>[7x]MRWILFILFCLLGAPAHAVSIPGVTTTTTTDSTTEPAPEPDIEQKKAAYGALADVLDNDTSRKELIDQLRT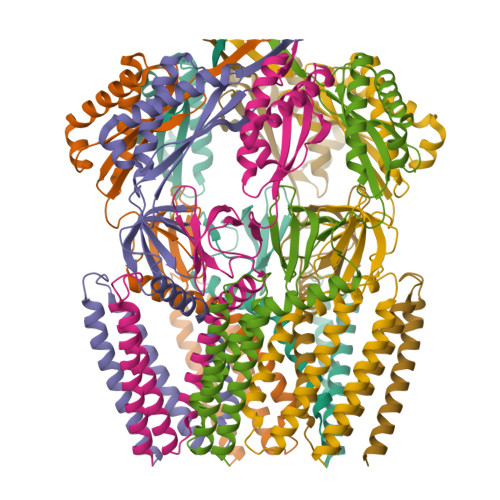VAATPPAEPVPKIVPPTLVEEQTVLQKVTEVSRHYGEALSARFGQLYRNITGSPHKPFNPQTFSNALTHFSMLAVLVFGFYWLIRLCALPLYRKMGQWARQKNRERSNWLQLPAMIIGAFIIDLLLLALTLFVGQVLSDNLNAGSRTIAFQQSLFLNAFALIEFFKAVLRLIFCPNVAELRPFTIQDESARYWSRRLSWLSSLIGYGLIVAVPIISNQVNVQIGALANVIIMLCMTVWALYLIFRNKKEITQHLLNFAEHSLAFFSLFIRAFALVWHWLASAYFIVLFFFSLFDPGNSLKFMMGATVRSLAIIGIAAFVSGMFSRWLAKTITLSPHTQRNYPELQKRLNGWLSAALKTARILTVCVAVMLLLSAWGLFDFWNWLQNGAGQKTVDILIRIALILFFSAVGWTVLASLIENRLASDIHGRPLPSARTRTLLTLFRNALAVIISTITIMIVLSEIGVNIAPLLAGAGALGLAISFGSQTLVKDIITGVFIQFENGMNTGDLVTIGPLTGTVERMSIRSVGVRQDTGAYHIIPWSSITTFANFVRGIGSVVANYDVDRHEDADKANQALKDAVAELMENEEIRGLIIGEPNFAGIVGLSNTAFTLRVSFTTLPLKQWTVRFALDSQVKKHFDLAGVRAPVQTYQVLPAPGATPAEPLPPGEPTLLEHHHHHH> MITMKDIIREGNPTLRAVAE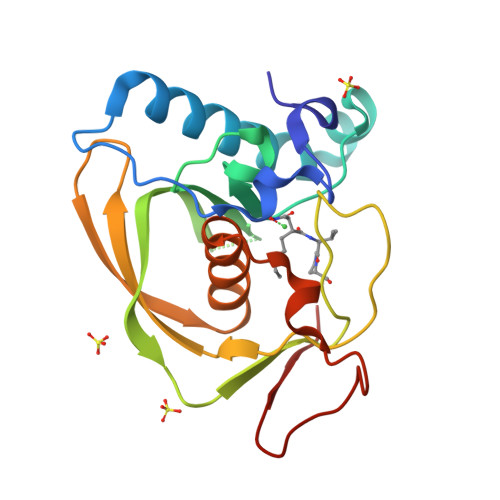EVPVPITEEDRQLGEDMLTFLKNSQDPVKAEELQLRGGVGLAAPQLDISKRIIAVHVPSNDPENETPSLSTVMYNPKILSHSVQDVCLGEGEGCLSVDRDVPGYVVRHNKITVSYFDMAGEKHKVRLKNYEAIVVQHEIDHINGIMFYDHINKENPFALKEGVLVIEL> MSERAPLVIIGTGLAGYNLAREWRKLDGETPLLMITADDGRSYSKPMLSTGFSKNKDADGLAMAEPG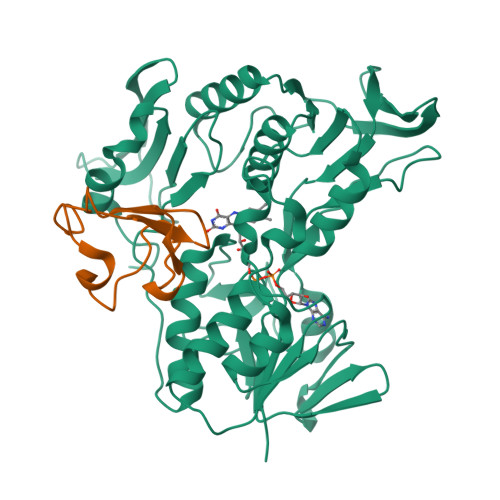AMAEQLNARILTHTRVTGIDPGHQRIWIGEEEVRYRDLVLAWGAEPIRVPVEGDAQDALYPINDLEDYARFRQAAAGKRRVLLLGAGLIGCEFANDLSSGGYQLDVVAPCEQVMPGLLHPAAAKAVQAGLEGLGVRFHLGPVLASLKKAGEGLEAHLSDGEVIPCDLVVSAVGLRPRTELAFAAGLAVNRGIVVDRSLRTSHANIYALGDCAEVDGLNLLYVMPLMACARALAQTLAGNPSQVAYGPMPVTVKTPACPLVVSPPPRGMDGQWLVEGSGTDLKVLCRDTAGRVIGYALTGAAVNEKLALNKELPGLMA;> MRKWQCVVCGFIYDEALGLPEEGIPAGTRWEDIPADWVCPDCGVGKIDFEMIEIA>GAMAPTPTDKHGGSDTRCPLMVKILDAVKGTPAGSVALKVSQKTADGGWTQIATGVTDATGEIHNLITEQQFPAGVYRVEFDTKAYWTNQGSTPFHEVAEVVFD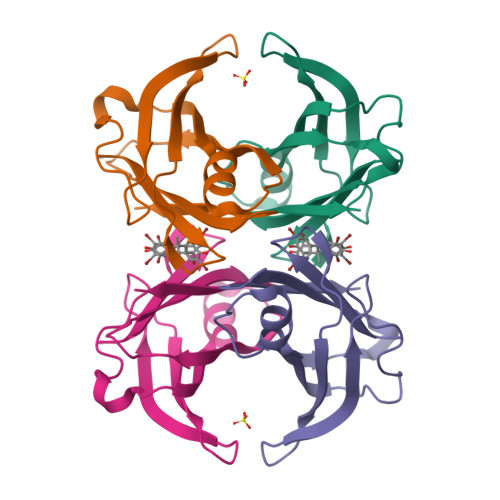AHPEGHRHYTLALLLSPFSYTTTAVVSSVHE[2x]>MDVSHHHHHHGMATARPAKARNEGQWALGHREPLNANEELKKAGNPLDVRERIENIYAKQGFDSIDKTDLRGRFRWWGLYTQREQGYDG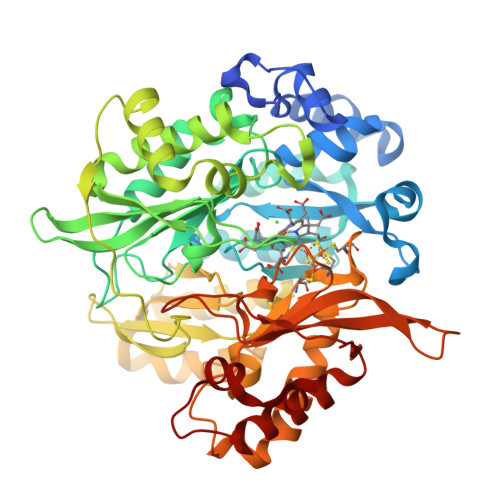TWTGDDNIDKLEAKYFMMRVRCDGGALSAAALRTLGQISTEFARDTADISDRQNVQYHWIEVENVPEIWRRLDDVGLQTTEACGDCPRVVLGSPLAGESLDEVLDPTWAIEEIVRRYIGKPDFADLPRKYKTAISGLQDVAHEINDVAFIGVNHPEHGPGLDLWVGGGLSTNPMLAQRVGAWVPLGEVPEVWAAVTSVFRDYGYRRLRAKARLKFLIKDWGIAKFREVLETEYLKRPLIDGPAPEPVKHPIDHVGVQRLKNGLNAVGVAPIAGRVSGTILTAVADLMARAGSDRIRFTPYQKLVILDIPDALLDDLIAGLDALGLQSRPSHWRRNLMACSGIEFCKLSFAETRVRAQHLVPELERRLEDINSQLDVPITVNINGCPNSCARIQIADIGFKGQMIDDGHGGSVEGFQVHLGGHLGLDAGFGRKLRQHKVTSDELGDYIDRVVRNFVKHRSEGERFAQWVIRAEEDDLR[2x]> GAMEADLSEPFSLTEVQTAYMLGRNPQFELSGISPQTYFEYETELDIARLSRSFQKVIQRHPMLRAVILPEGKQQILRDVPEYEIEVESLVSMPPEKQAARLREERSRMIDHVFPLGQWPLFELKAFQLQEHTYLLCFRYDALLMDGASMNLVGQDLMHYYHQPDAQLPPLSFTFQDYMHIYDDMKRGTEYETAKAYWTNKLPDFPPAPSLLLAKDPAEIGTPNFQSLTTIITKDKWLKLRRLAQDKQVTPSALLCTVYGEVLAFWSNQRRLAINLTVFNRYPVHDEVEQIVGDFTSLILLDMDMDQKQPFFTKVEQTQSTLLDGLEHRHYDGVEFIRDYTRYHQMRPKAVMPIVFTSMLAGAGAFAWEEIGSLRHIHARTPQVYLDNVVIEKNGELLVSWNYVEELFD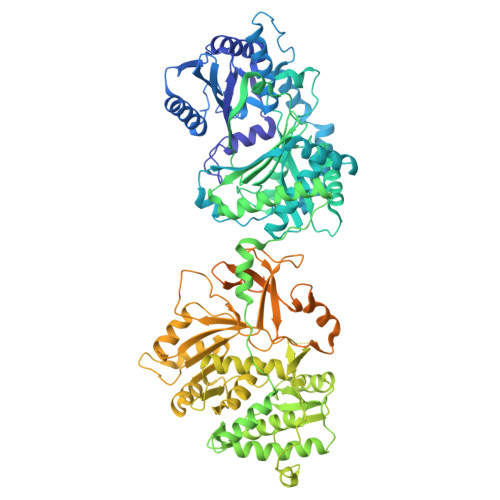AEVMESMFTQFVELLDQLVEQGDINPLRISQKDYALIDQYNATAEPIPAATLHQLFIDQAQRTPDQVAVVFEQEWLTYSELDQRSNQVARFLQSRGIGRGDRVGVLAKRQVETIINLMAVLKAGAAYVPIDPDHPYERQTYILENSSCKILLDSDLYETMEISSYADGDLTPVAEPEDTAYVIYTSGSTGRPKGVIITHQAASNTIQDINRKFEVNEEDRIIGISSMCFDLSVYDIFGTLSAGATLVMIRDPRDMRELVRTVERRGITIWNTVPAIMDLALDHVGSHFENISLRLVLLSGDWIPLPLPAKINRHFPVADVISLGGATEASIWSIYWPIEQVEANWKSIPYGKPLANQTYYVLNYDQKMCPVGVIGDLYIGGAGLAQGYLNDDQKTKDAFIMHPEFGPIYKTGDCGRMRPEGYIEFLGRQDYQVKIQGYRVELEEISHCLLTYPDVDQAVVIDQTDERGMKFLVGYVVAQQEIDEKALRKHLMEHLPEYMIPAHLVHLEQLPLTPNGKLDRKALPVPKKQRNAEKFVAPQAGLEKILASVWQEVLNVEQIGANDHFFALGGDSIKAIQVSARLFVQGYHLDTKSLFEFPVLRDVARTIKKLAAAENLYFQ>[5x]MFSGIKGPNPSDLKGPELRILIVHARYNLQAIEPLVKGAVETMIEKHDVKLENIDIESVPGSWELPQGIRASIARNTYDAVIGIGVLIKGSTMHFEYISEAVVHGLMRVG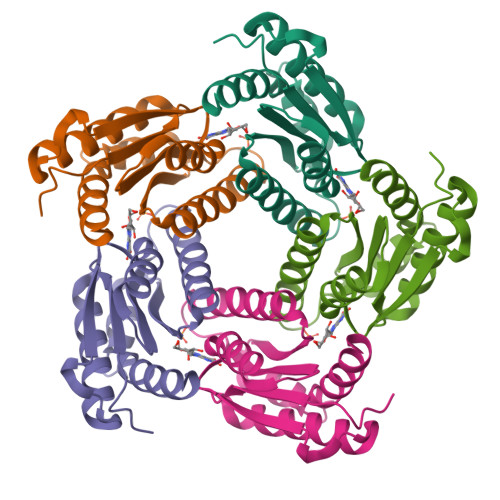LDSGVPVILGLLTVLNEEQALYRAGLNGGHNHGNDWGSAAVEMGLKALY> MTLATKVFKLSFKTPVHFGKKRLSDGEMTITADTLFSALFIETLQLGKDTDWLLNDLIISDTFPYENELYYLPKPLIKIDSKEEDNHKAFKKLKYVPVHHYNQYLNGELSAEDATDLNDIFNIGYFSLQTKVSLIAQETDSSADSEPYSVGTFTFEPEAGLYFIAKGSEETLDHLNNIMTALQYSGLGG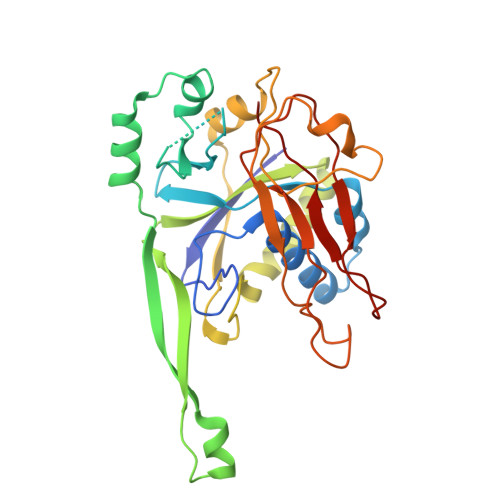KRNAGYGQFEYEIINNQQLSKLLNQNGKHSILLSTAMAKKEEIESALKEARYILTKRSGFVQSTNYSEMLVKKSDFYSFSSGSVFKNIFNGDIFNVGHNGKHPVYRYAKPLWLEV>MELIKGQALFLELDKKDFLSLKNNDKNIPTFAHPKNQEKILAIFSLPYKNPPQNTKLIAFYKDKKEEIFIKTLEGNYKSEKLQVENKKIFPPKTIQERIAKELKEANAIYSSYTPKALFNGAFNIPLNSFITSDFGKARTFNEKVASYHSGTDFRAATGTPIYAANSGVVKIAKDRYFAGNSVVIDHGFGIYSQYYALSKIDVKVGQKIKKGELIGLSGASGRVSGPHLHFGILAGGKQVDPLDFVSKFNAIFQLEHHHHHH[3x]

We have described herein the reactions and the structure of Pgp3, a Csd protein of C. jejuni. This enzyme turns over the cell-wall peptidoglycan by both the d,d-endopeptidase and d,d-carboxypeptidase activities, as documented by mass spectrometric characterization of the requisite reactions with synthetic cell-wall fragments. The Pgp3 monomer is structurally divided into four regions: the N-terminal domain (NTD, residues 21–95), a flexible linker (residues 96–147), the LytM domain (residues 148–259), and the C-terminal helix (residues 260–273). The Pgp3 LytM domain contains a highly conserved tetrahedral Zn2+-ion-binding motif (H168xxxD172 and HxH249).

We decided to mutate His216 and His247 individually to alanine in order to abrogate the binding of tartrate or citrate at the active site and impair catalysis too. In the case of the H216A variant, tartrate was sometimes observed in the closed form crystal structure; hence, only the H247A variant was pursued further. The structures are: (i) tartrate-bound wild type (WT) (open form), (ii) citrate-bound WT (two structures, closed form), (iii) H216A mutant (open form), (iv) H216A mutant with tartrate (closed form), (v) H247A mutant (open form), (vi) H247A mutant with pentapeptide 1, Ac-l-Ala1-γ-d-Glu2-mDAP3-d-Ala4-d-Ala5 (open form), and (vii) H247A mutant with crosslinked muramyl tetra-tri peptide 2, NAM-l-Ala1-γ-d-Glu2-mDAP3-d-Ala4-mDAP3-γ-d-Glu2-Ala1-NAM (open form). Since crystals of Pgp3 contained one or three subunits in the asymmetric unit of WT and variants (H216A and H247A, both discussed later) depending on the space group, we analyzed the oligomeric states of the WT and variant Pgp3 in solution using size-exclusion chromatography with multi-angle light scattering (SEC-MALS) experiments. Crystals of Pgp3 could only be produced in the presence of either tartrate or citrate molecules. Both molecules bound to the active site of Pgp3 via several hydrogen bonds and salt-bridge interactions between the carboxyl groups of tartrate or citrate and the Zn2+ ion.>MSKHSISLGGQLEDNWRTLSEVLETATKHNNHGITYIRNDATEYFQSYQDLYQDALVILNGLEQKGIKLGHKVILQIAKNQDFIPALWACFLGGIIPVPLTVAPSYDLENSAVKKLEN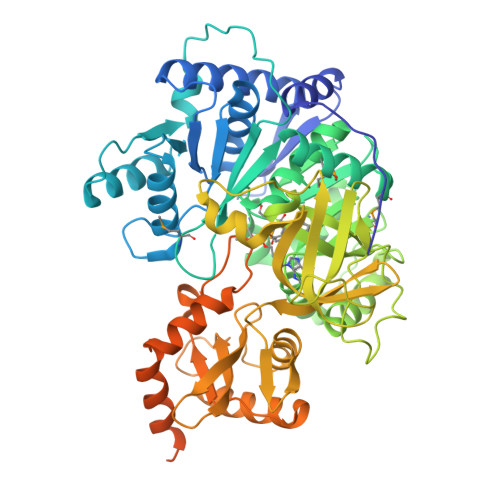VWKILDNPLILSDSELITEIEKLGTYSHLEGWQVISVNELRKAPSKIEQLPILDPQDAALLLFTSGSTGMPKGVILTHHNILSMTAGTVVMNHFTQQEVTLNWMPLDHVGAIVFLGIMAVDLACDQIHVPMELVLRQPLQWLELIQKHQVSISWSPNFAFSLINQQAEELKHVSYNLSSMKFLVNAGEQVSVKTIRLFLEILEKHQLQERAIKPAFGMTESCSGITWSAGLSKNELTEENSFVSLGKPIPGATIRIVDQENNPLPEREIGRLQIQGNSVTKGYYNNNELNQEVFQEGWFTTGDLGYLSKGELFITGREKQEIIINGVNYFAHELETTIEELEGVKVSYTAAFAVFDQSRETDLLIITFSPESEQFEQGIKVVRKIRSHVTQKFGIAPAYVIPLERNLVPKTSIGKVQKSKLKKDFEQGLFSSRIQEIDQYLAKERQKNQTLPQSENERQIAAVWSEVLQLTSVGLEDNFFELGGHSIHLIRVQNELEKLFNRQLSLAEMFKNPTVATLARFLSEE[2x]> HHHHHHSEMQDLYPSRQRADAEMR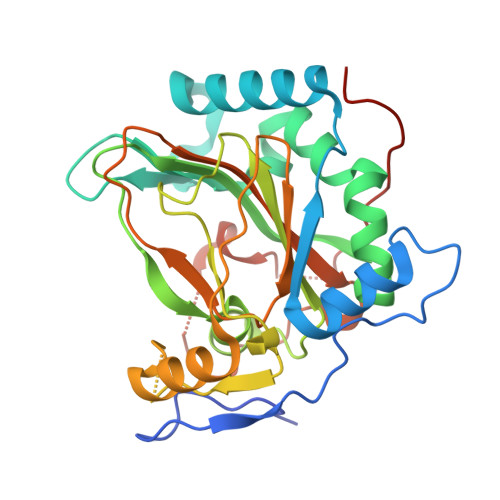PRLDPVVHSEWTNDAPISARQAAAFDRDGYIVLEDIFSADEVAFLQKAAGNLLADPAALDADTIVTEPQSNEIRSIFEIHAQSPVMARLAADARLADVARFLLGDEVYIHQSRLNYKPGFKGREFYWHSDFETWHVEDGMPRMRALSMSVLLAENTPHNGPLMVIPGSHRTYLTCVGETPDDHYLSSLKKQEYGVPDEESLAELAHRHGIVAPTGKPGTVILFDCNLMHGSNGNITPFPRANAFLVYNAVSNRLEKPFGVEKPRPWFLARRGEPAALRVERGPLVETVPA>MNHK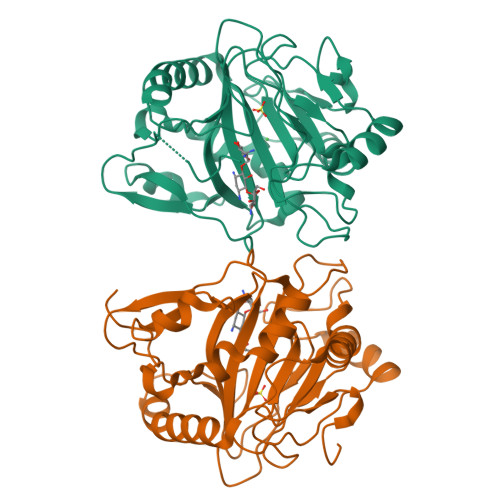VHHHHHHIEGRHMALAAPPGELTLALTPDDKTLDPASLDRALAILAEHGILVLTGMLRTRLTDQLRTAMLDDLPEVLRQQDVPTNFVPGHVQQDPPVRESLLFPDVLLNPVVYQITHAVLGADARNAVYSGNMNLPGSHEQPVHLDEPHLWPGISHPPYCLCVDVPLIDFTLENGSTEYWPGSHVLNPDECYDERGCVLPAELERRRAVAPPVRFPIPVGSVVIRDGRLWHRGVPNLSAAPRPLLAMTHYTEWFDMPPIQLPDTVKSWVDGSDRHTHAHFVAGDVDHLTGDHPFAVR[6x]[(2R,3S,5R)-5-(6-amino-8-phenyl-9H-purin-9-yl)-3-hydroxyoxolan-2-yl]methyl [(2R,3S,4S,5R)-3,4,5-trihydroxyoxolan-2-yl]methyl dihydrogen diphosphate 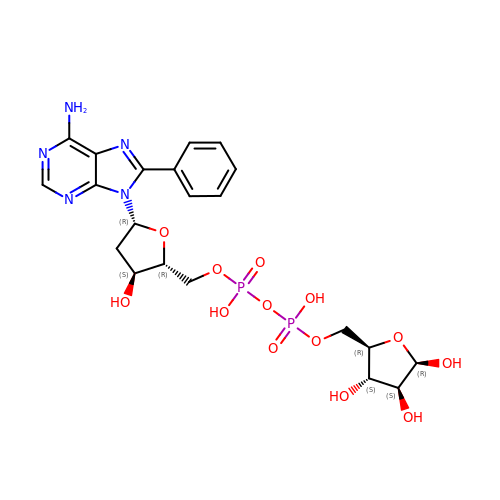(non-preferred name) | C21 H27 N5 O13 P2 | HDAKJMFIHMDGRC-SXAIUVOJSA-N>SKPKQPPDASPANLLTSLVRAHLDSGPSTAKLDYSKFQELVLPHFGKEDAGDVQQFYDLLSGSLEVIRKWAEKIPGFAELSPADQDLLLESAFLELFILRLAYRSKPGEGKLIFCSGLVLHRLQCARGFGDWIDSILAFSRSLHSLLVDVPAFACLSALVLITDRHGLQEPRRVEELQNRIASCLKEHVAAVAGEPQPASCLSRLLGKLPELRTLCTQGL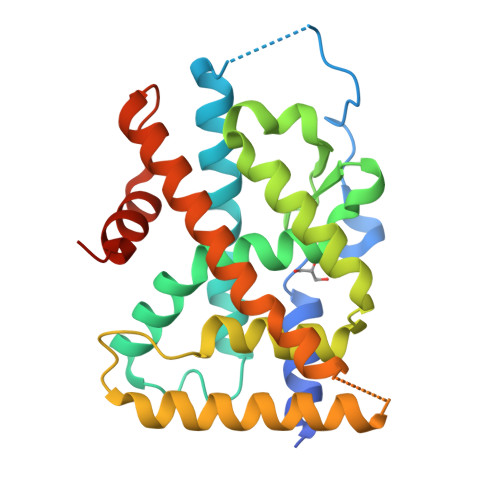QRIFYLKLEDLVPPPPIIDKIFMDTLPFLEHHHHHH[2x]> SIDSALNWDGEMTVTRFDSMTGAHFVIRLDSTQLGPAAGGTRAAQYSQLADALTDAGKLAGAMTLKMAVSNLPMGGGKSVIALPAPRHSIDPSTWARILRIHAENIDKLSGNYWTGPDV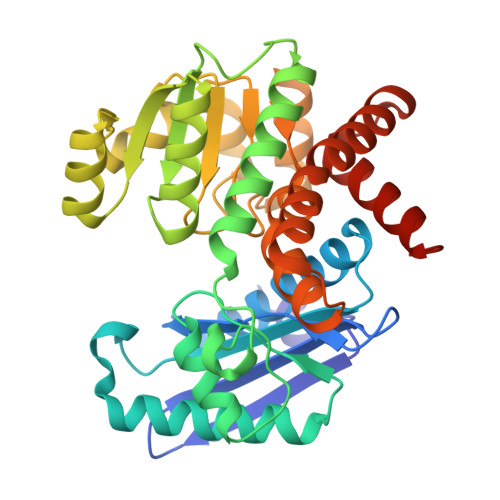NTNSADMDTLNDTTEFVFGRSLERGGAGSSAFTTAVGVFEAMKATVAHRGLGSLDGLTVLVQGLGAVGGSLASLAAEAGAQLLVADTDTERVAHAVALGHTAVALEDVLSTPCDVFAPCAMGGVITTEVARTLDCSVVAGAANNVIADEAASDILHARGILYAPDFVANAGGAIHLVGREVLGWSESVVHERAVAIGDTLNQVFEISDNDGVTPDEAARTLAGRRAREASTTTATA>PVVIKTEGPAWTPLEPKLITRLADTVRTKGLRSPITMAEVEALMSSPLLPHDVTNLMRVILGPAPYALWMDAWGVQLQTVIAAATRDPRHPANGQGRGERTNLNRLKGLADGMVGNPQGQAALLRPGELVAITASALQAFREVARLAEPAGPWADIMQGPSESFVDFANRLIKAVEGSDLPPSARAPVIIDCF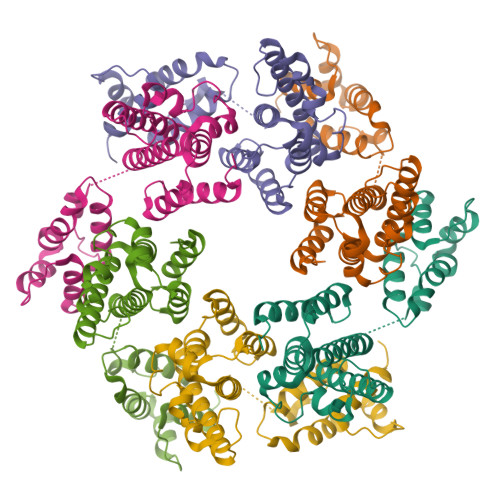RQKSQPDIQQLIRTAPSTLTTPGEIIKYVLDRQKTA[6x]> HHMDEEYDVIVLGTGLTECILSGIMSVNGKKVLHMDRNPYYGGESSSITPLEELYKRFQLLEGPPETMGRGRDWNVDLIPKFLMANG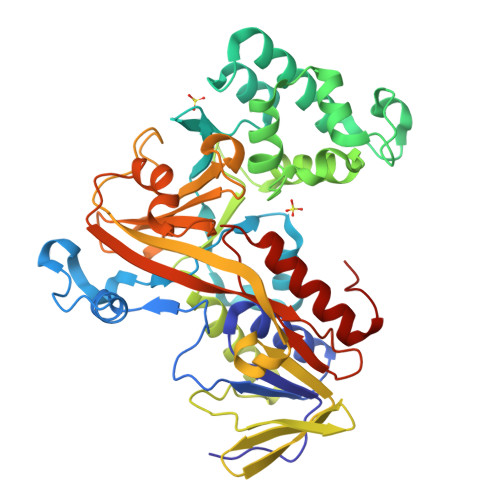QLVKMLLYTEVTRYLDFKVVEGSFVYKGGKIYKVPSTETEALASNLMGMFEKRRFRKFLVFVANFDENDPKTFEGVDPQNTSMRDVYRKFDLGQDVIDFTGHALALYRTDDYLDQPCLETINRIKLYSESLARYGKSPYLYPLYGLGELPQGFARLSAIYGGTYMLNKPVDDIIMENGKVVGVKSEGEVARCKQLICDPSYVPDRVRKAGQVIRIICILSHPIKNTNDANSCQIIIPQNQVNRKSDIYVCMISYAHNVAAQGKYIAIASTTVETTDPEKEVEPALGLLEPIDQKFVAISDLYEPIDDGSESQVFCSCSYDATTHFETTCNDIKDIYKRMAGSAFDF> NGDRLYKADSRPPDEIKRSGGLMPRGHNEYFDRGTQMNINLYDHARGTQTGFVRYDDGYVSTSLSLRSAHLAGQSILSGYSTYYIYVIATAPNMFNVNDVLGVYSPHPYEQEVSALGGIPYSQIYGWYRVNFGVIDERLHRNREYRDRYYRNLNIAPAE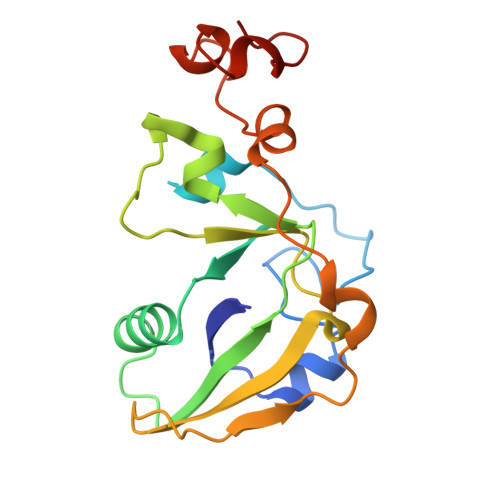DGYRLAGFPPDHQAWREEPWIHHAPQGCGNSS> GEVVDCHLSDMLQQLHSVNASKPSERGLVRQEEAEDPACIPIFWVSKWVDYSDKYGLGYQLCDNSVGVLFNDSTRLILYNDGDSLQYIERDGTESYLTVSSHPN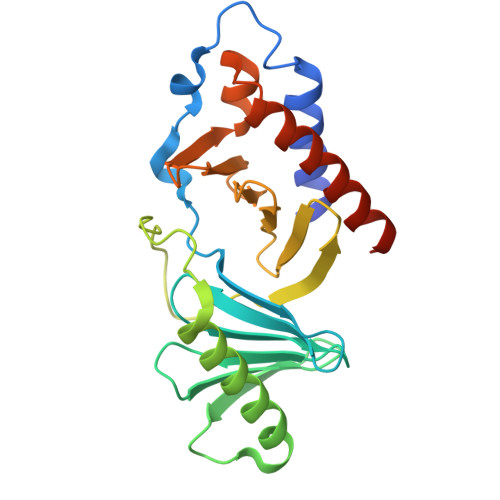SLMKKITLLKYFRNYMSEHLLKAGANITPREGDELARLPYLRTWFRTRSAIILHLSNGSVQINFFQDHTKLILCPLMAAVTYIDEKRDFRTYRLSLLEEYGCCKELASRLRYARTMVDKLLSSRSASNRLKAS> MGSDKIHHHHHHENLYFQGADWKVGIQTWTFHNLTLMETLDKTQQLGMGYAEAFFFQELGAPFPKETYLNYDLSDDNCALLRHEFKIRGIKPIAFGVASYGTNEEWDKFFAFAHKIGAHIVTVEPELNQLDYIESLAKKYDMEVAIHNHPSPCIYASAEVVEKALKGRSPLMGVCADIGHWKRVGEDPLKNLQKLSGRIK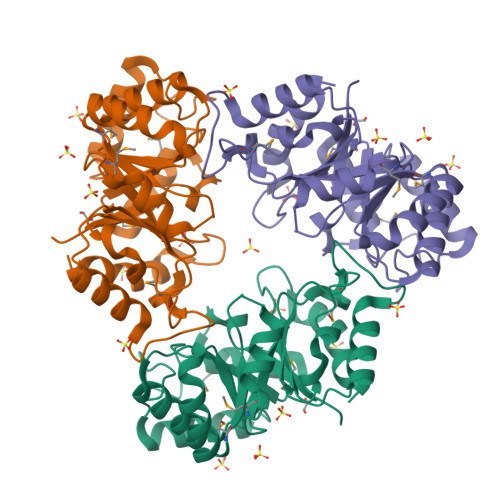VAHLKDLTDKMEDATWGTGILPVKAFVNELKRQHFNGLISIEYDDFKSDIQEIRNSLEFLQKCSK>[2x]MNHKVHHHHHHMLIILTGLPGVGKSTFSKNLAKILSKNNIDVIVLGSDLIRESFPVWKE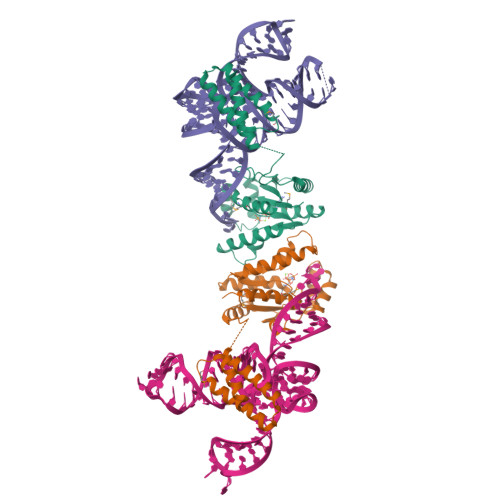KYEEFIKKSTYRLIDSALKNYWVIVDDTNYYNSMRRDLINIAKKYNKNYAIIYLKASLDVLIRRNIERGEKIPNEVIKKMYEKFDEPGKKYKWDEPFLIIDTTKDIDFNEIAKKLIEKSKEIPKFYVLEENKNKNNNISDKIDKETRKIVSEYIKSKKLDKDKIKEVVELRKEFLKKIKKMEEVDADRVLKEFKDLLNSY> LPTSNPAQELEARQLERTTRDDLINGNSASCADVIFIFARGSTETGNLGTLGPSIASNLESAFGKDGVWIQGVGGAYRATLGDNALPRGTSSAAIREMLGLFQQANTKCPDATLIAGGYSQGAALAAASIEDLDSAIRDKIAGTVLFGYTKNLQNRGRIPNYPADRTKVFCNTGDLVCTGSLIVAAPH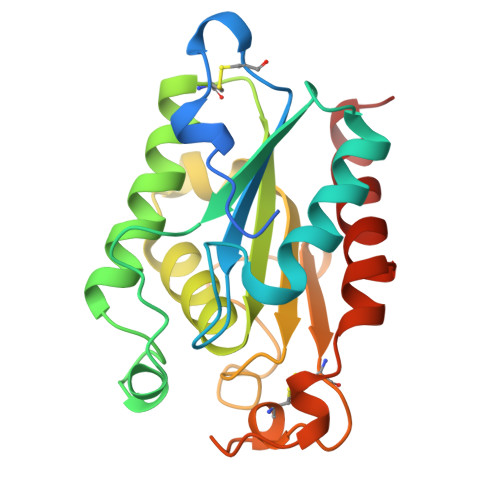LAYGPDARGPAPEFLIEKVRAVRGSA> MNSPISPIETVPVKLKPGMDGPKVKQWPLTEEKIKALVEICTEMEKEGKISKIGPENPYNTPVFAIKKKDSTKWRKLVDFRELNKRTQDFWEVQLGIPHPAGLKKKKSVTVLDVGDAYFSVPLDEDFRKYTAFTIPSINNETPGIRYQYNVLPQGWKGSPAIFQSSMTKILEPFRKQNPDIVICQYMDDLYVGSDLEIGQHRTKIEELRQHLLRWGLTTPDKKHQKEPPFLWMGYELHPDKWTVQPIVLPEKDSWTVNDIQKLVGKLNWASQIYPGIKVRQLCKLLRGTKALTEVIPLTEEAELELAENREILKEPVHGVYYDPSKDLIAEIQKQGQGQWTYQIYQEPFKNLKTGKYARMRGAHTNDVKQL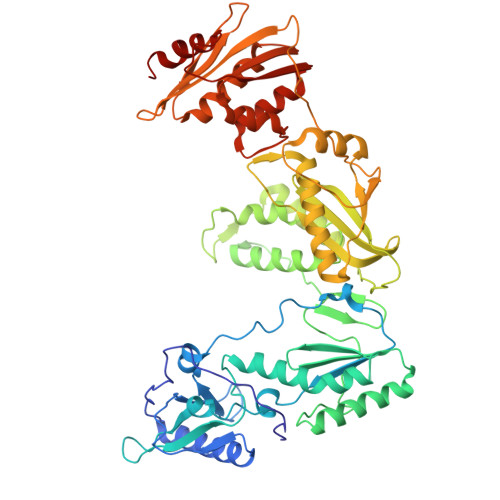TEAVQKITTESIVIWGKTPKFKLPIQKETWETWWTEYWQATWIPEWEFVNTPPLVKLWYQLEKEPIVGAETFYVDGAANRETKLGKAGYVTNRGRQKVVTLTDTTNQKTELQAIYLALQDSGLEVNIVTDSQYALGIIQAQPDQSESELVNQIIEQLIKKEKVYLAWVPAHKGIGGNEQVDKLVSAGIRKVL> MAFSVLNWDQVSRLHEVLTEVVPIHGRGNFPTLEITLKDIVQTVRSRLEEAGIKVHDVRLNGSAAGHVLVKDN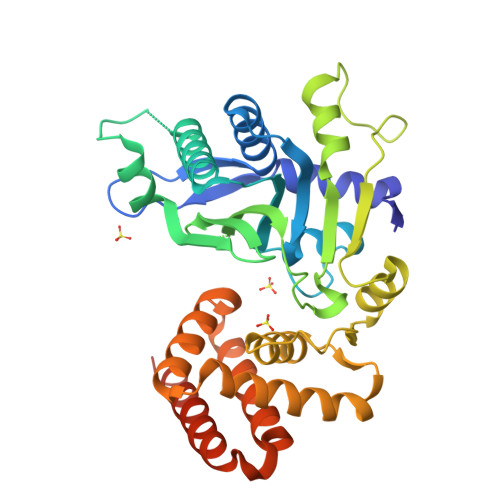GLGCKDLDLIFHVALPTEAEFQLVRDVVLCSLLNFLPEGVNKLKISPVTLKEAYVQKLVKVCTDTDRWSLISLSNKNGKNVELKFVDSIRRQFEFSVDSFQIILDSLLFFYDCSNNPISEHFHPTVIGESMYGDFEEAFDHLQNRLIATKNPEEIRGGGLLKYSNLLVRDFRPTDQEEIKTLERYMCSRFFIDFPDILEQQRKLETYLQNHFAEEERSKYDYLMILRRVVNESTVCLMGHERRQTLNLISLLALRVLAEQNIIPSATNVTCYYQ Hexameric MCM rings act as the replicative DNA helicase, encircling the leading strand DNA template at the replication fork. Each Mcm subunit contains three domains. The N-terminal domain (MCMN) possesses an OB (oligonucleotide/oligosaccharide binding)-fold and usually a zinc-binding motif. The MCM complexes of several archaeal organisms consist of six identical subunits and have provided powerful models to investigate the atomic details of MCM structure.

The structure is similar to those of MtMCMN and SsoMCMN with three subdomains: a largely helical subdomain A; a Zn-binding subdomain B; and an OB-fold subdomain C. The central pore of the PfMCMN hexameric ring is oval-shaped with a variable diameter around the ring reflecting a significant deviation from pure sixfold symmetry. The RMSD of the C-subdomain Cα-positions from the sixfold permutation is 3.03 Å and 1.45 Å for hexamers 1 and 2, respectively. The ssDNA circles the interior of the PfMCMN ring in a plane perpendicular to the central channel. When viewed from the C-terminal side of the complex, the 5′ to 3′ direction of the bound ssDNA proceeds clockwise around the channel. The structure reveals that the individual MCM subunits do not all simultaneously participate in ssDNA binding. The subunits that interact with DNA use a consistent binding mode with four nucleotides per subunit. DNA-binding is consistently observed at the first subunit if this distance is less than 7.5 Å, and it is not observed if this distance exceeds 8.4 Å. The most significant interactions between PfMCMN and ssDNA involve two adjacent arginines, R124 and R186, that project from the β-barrel of the OB-fold towards the ring interior. The DNA-binding consists predominantly of interactions with the sugars and bases rather than the backbone phosphates.

>[12x]SVDREEMIERFANFLREYTDEDGNPVYRGKITDLLTITPKRSVAIDWMHLNSFDSELAHEVIENPEEGISAAEDAIQIVLREDFQREDVGKIHARFYNLPETLMVKDIGAEHINKLIQVEGIVTRVGEIKPFVSVAVFVCKDCGHEMIVPQKPYESLEKVKKCEQCGSKNIELDVNKSSFVNFQSFRIQDRPETLKGGEMPRFIDGILLDDIVDVALPGDRVIVTGILRVVLEKREKTPIFRKILEVNHIEPVSKEI~{O}1-[(2~{R})-2-ethylhexyl] ~{O}2-[(2~{S})-2-ethylhexyl] benzene-1,2-dicarboxylate 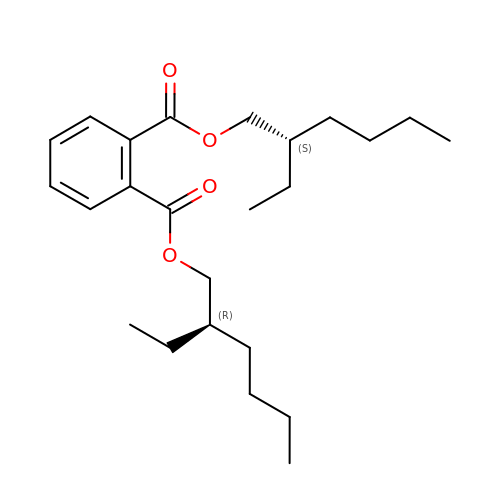| C24 H38 O4 | BJQHLKABXJIVAM-BGYRXZFFSA-N> QEALEERARNELSLTRPGETFY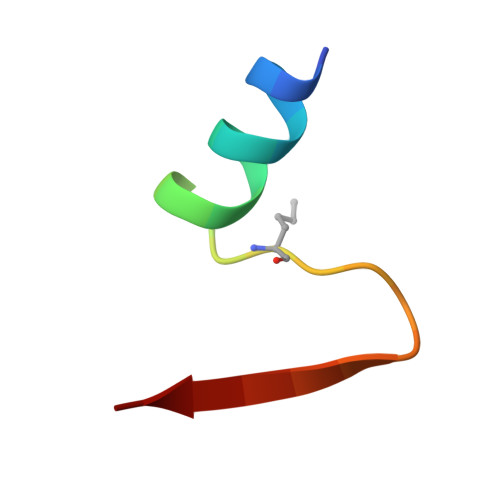RL> GHMQETQAVEAGEKTVEQFVQALNKGDYNKAAEMTSKKAANKSALSEKEILDKYQNIYGAADVKGLQISNLKVDKKDDSTYSFSYKAKMNTSLGELKDLSYKGTLDRNDGQTTINWQPNLVFPEMEGNDKVSLTTQE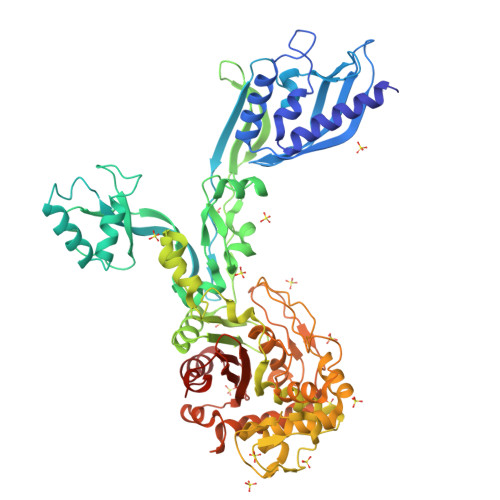AARGNIIDRNGEPLATTGKLKQLGVVPSKLGDGGEKTANIKAIASSFDLTEDAINQAISQSWVQPDYFVPLKIIDGATPELPAGATIQEVDGRYYPLGEAAAQLIGYVGDITAEDIDKNPELSSNGKIGRSGLEMAFDKDLRGTTGGKLSITDADGVEKKVLIEHEVQNGKDIKLTIDAKAQKTAFDSLGGKAGSTVATTPKTGDLLALASSPSYDPNKMTNGISQEDYKAYEENPEQPFISRFATGYAPGSTFKMITAAIGLDNGTIDPNEVLTINGLKWQKDSSWGSYQVTRVSDVSQVDLKTALIYSDNIYMAQETLKMGEKKFRIGLDKFIFGEDLDLPISMNPAQISNEDSFNSDILLADTGYGQGELLINPIQQAAMYSVFANNGTLVYPKLIADKETKDKKNVIGETAVQTIVPDLREVVQDVNGTAHSLSALGIPLAAKTGTAEIKEKQDVKGKENSFLFAFNPDNQGYMMVSMLENKEDDDSATKRASELLQYLNQNYQ>[3x]MATKAARAPRTVLPFEAMPQHPGNRWLRLLQIWREQGYEHLHLEMHQTFQELGPIFRYNLGGPRMVCVMLPEDVEKLQQVDS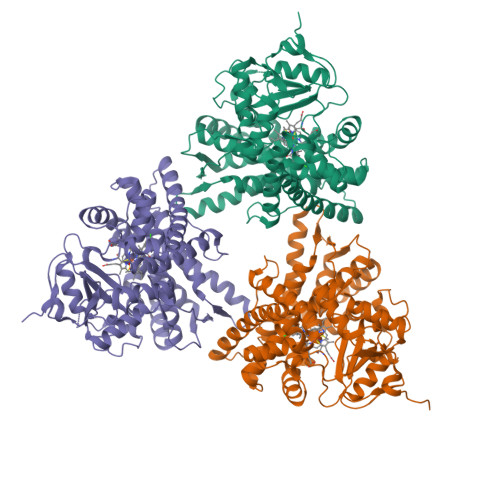LHPCRMILEPWVAYRQHRGHKCGVFLLNGPEWRFNRLRLNPDVLSPKAVQRFLPMVDAVARDFSQALKKKVLQNARGSLTLDVQPSIFHYTIEASNLALFGERLGLVGHSPSSASLNFLHALEVMFKSTVQLMFMPRSLSRWISPKVWKEHFEAWDCIFQYGDNCIQKIYQELAFNRPQHYTGIVAELLLKAELSLEAIKANSMELTAGSVDTTAFPLLMTLFELARNPDVQQILRQESLAAAASISEHPQKATTELPLLRAALKETLRLYPVGLFLERVVSSDLVLQNYHIPAGTLVQVFLYSLGRNAALFPRPERYNPQRWLDIRGSGRNFHHVPFGFGMRQCLGRRLAEAEMLLLLHHVLKHFLVETLTQEDIKMVYSFILRPGTSPLLTFRAINGGRHHHHHH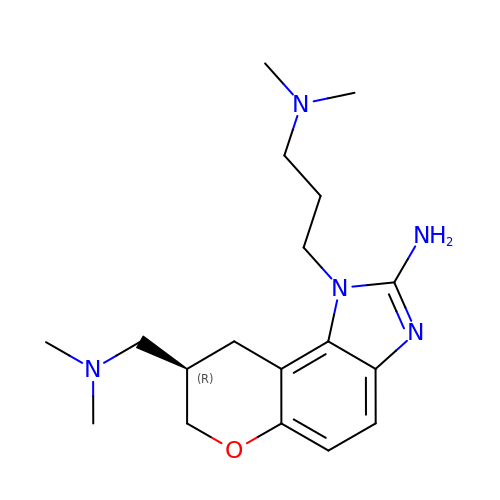(8R)-8-[(dimethylamino)methyl]-1-[3-(dimethylamino)propyl]-1,7,8,9-tetrahydrochromeno[5,6-d]imidazol-2-amine | C18 H29 N5 O | HTUXJUVSTFSWOD-CYBMUJFWSA-N> ASMTGGQQMGRGSGPMLIEFNIPVDLKLVEQQNPKVKLGGRYTPMDGASVHKMALLVPFRDRFEELLQFVPHMTAFLKRQGVAHHIFVLNQVDRFRFNRASLINVGFQFASDVYDYIAMHDVDLLPLNDNLLYEYPSSLGPLHIAGPKLHPKYHYDNFVGGILLVRREHFKQMNGMSNQYWGWGLENDEFFVRIRDAGLQVTRPQNIKTGTNDTFSHIHNRYHRKRDTQKCFNQKEMTRKRDHKTGLDNVKYKILKVHEMLIDQVPVT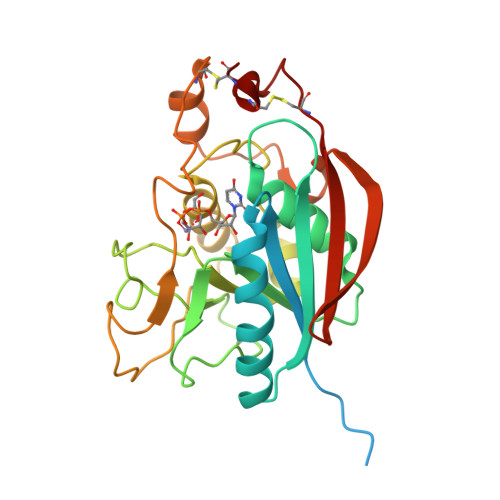ILNILLDCDVNKTPWCDCS Bacterial homologous lysine and arginine decarboxylases play major roles in the acid stress response, physiology, antibiotic resistance and virulence. Inducible AAT-fold basic amino acid decarboxylases (LAOdcs) have been studied since the early 1940s1,2 because of the link between their enterobacterial pathogenicity in humans and their ability to overcome the aggressive pH environments and oxygen limitation in our gastrointestinal tract. These enzymes decarboxylate either Lysine (LdcI, also called CadA), Arginine (Adc or AdiA) or Ornithine (OdcI or SpeF) into corresponding polyamines while consuming protons and producing CO2, thereby buffering the bacterial cytosol and the extracellular medium to promote bacterial survival under acid stress conditions. Here we show that the Adc from a multidrug-resistant human pathogen Providencia stuartii massively polymerises into filaments whose cryo-EM structure reveals pronounced differences between Adc and LdcI assembly mechanisms. Like all proteobacterial LAOdcs, the P. stuartii Adc monomer is organized in three different structural parts.

In the decameric double ring, two monomers form a C2-symmetric dimer, which represents the basic unit of the structure and forms a decameric assembly through strong inter-ring contacts between adjacent dimers. This type of dimerisation is typical for proteobacterial LAOdcs and for pyridoxal 5′-phosphate (PLP)-dependent enzymes in general, and leads to a completion of the active sites of each monomer buried into a cleft at the dimer interface. The N-terminal wing domain protrudes into the centre of the double ring and is involved in stabilisation of the decamer assembly though inter-dimer contacts (residues 1-139). Preceded by a short linker region (residues 140-192), the central core part contains the covalently-bound PLP cofactor and is composed of a PLP-binding domain (residues 193-439) and an aspartate aminotransferase-like domain (residues 440-608). The C-terminal domain (residues 609-758), located at the decamer periphery, partially constitutes an entry channel into the active site. The Root-Mean-Square Deviation between P. stuartii and E. coli Adc monomers is 0.52 Å (over 4424 atoms), which illustrates their strong overall similarity. At the sequence level, the wing domains of the P. stuartii and the E. coli Adc proteins are the most different (52.14% identity) whereas the PLP-binding domain is the most conserved (77.33% identity). Although the exact residues involved in both dimerisation and decamerisation of the P. stuartii and E. coli Adcs differ, the buried surface area (BSA) and predicted ∆G upon decamerisation is similar for both proteins. In contrast, our Mass Photometry analysis of P. stuartii Adc indicates the presence of the decameric species at pH 5 and 6.5, whereas lower molecular weight species are detected at pH 8 but also unexpectedly at pH 4.

>[10x]MRALIVYTELTDKDSVISHAVARLASELNDEHVETVIIRDFEDGLAYIRSNTSIDCLLYGRDMSDRDEQIQAHRLITQLHRRQEDVPVFLLSDREEALVAFDRNMMEQVDEFAWILEDSADFIAGRVLAAIQRYRSQLLPPLMKSLIKYSDVHEYSWAAPGHQGGVGFTKTPAGRIYHDFFGENLFRTDIGIERVAVGSLLDHTGAFGECEKNAARIFGADQSYSVVVGTSGSNRTIMQACMTDDDVVVIDRNCHKSIEQGLILTGAKPVYMIPSRNRYGIIGPIYPKEMTPDAIKFKIAANPLTKGKVKQKPAYSVVTNCTYDGVCYNARKVQDLLDGSLDRIHFDEAWYGYARFNPLYRNHFAMRDEERTENEPTIFATHSTHKLLNALSQASFIHVRNGRNAIDFNRFNQAYLMHSTTSPLYAICASNDIAADMMDGNSGRSLTDEVIRESIDFRQSLAYLYKEFLNDDEWFFKPWNQEMVKDPATGKRYAFEDAPVELLMREQSCWVMHPEDKWHGFNDIPDNWAMLDPIKVSILAPGMGDDGKLLDTGVPAALVTAWLNHYGIVPTRTTDFQIMFLFSMGITKGKWGTLVNTLLSFKRHYDNNTALKKVLPEVVASAPEIYGEMGLRDLGDKMFAYLQKNNPGARLNQAYSQLPQVMMTPRDAYQQIVANRVEAVPVDQLMGRVAANSIIPYPPGIPMLLSGENFGDENSPHIHYLRSLQAWDSEFPGFEHETEGTEIIDGQYYVMCVKTCDE Furthermore, EmbB has been shown to play a key role in forming the characteristic terminal hexarabinofuranosyl motif of AG, which is the template for mycolylation. Together with the other Emb proteins (EmbA and EmbC), EmbB belongs to the glycosyltransferase C (GT-C) superfamily, whose structures comprises an N-terminal transmembrane domain and a C-terminal soluble domain located on the periplasmic side of the membrane. EmbB is observed as a dimer along with an acyl-carrier-protein (AcpM) associated with each protomer, thus forming a heterotetrameric EmbB2-AcpM2 complex. The EmbB protomers in the two states share common structural features which include two periplasmic domains (PDs) and 15 transmembrane helices (TMH) arranged into an approximately crescent-shaped bundle.

In this study, we have determined the structures of a substrate unbound EmbB2-AcpM2 complex in a presumed resting state and a donor DPA-bound pre-catalytic conformation which we define as the “active” state. The EmbB2-AcpM2 complex is captured in two states, one with C2-symmetry and the other that is asymmetric. Given their differences in composition and conformation, the two states are referred to as the asymmetric “donor-bound” active state and the symmetric “resting” state. Another structural rearrangement upon DPA binding, by comparing the structures of the two states, involves α6 in PL5, a short α helix that interacts with DPA, whereas in the resting state, this region is disordered. Considering that the bound DPA is the major composition difference between the two states, it is reasonable to speculate that the dramatic structural rearrangement of the enzyme complex in the active state occurs upon DPA binding, and is mediated by the induced disorder-to-helix transition of α6 at the dimer interface. When superimposing the EmbB protomer from the EmbB2 in its resting state onto the EmbB subunit of ethambutol-bound EmbA-EmbB complex, residues including the catalytic site D285 on EmbB2 were obsereved in the similar position. Thus it is possible the ethambutol inhibition mode on EmbB2 similar to that on EmbA-EmbB complex by inhibiting substrate binding. Notable shifting (2.9~4.0 A°) were observed on E313 on PL2 and H580 on PL6, likely due to ethambutol binding.

>[2x]MSGNMDEAVSGNMDEAVSAGKDVRIARWVATIAGLLGFVLSVSIPLLPVTQTTATLNWPQQGRLDNVTAPLISQAPLELTATVPCSVVRDLPPEGGLVFGTAPAEGRDAALNAMLVNVTETRVDVIVRNVVVASVNRDRVAGPDCQRIEITSNLDGTYADFVGLTQISGEDAGKLQRTGYPDPNLRPAIVGVFTDLTGPAPQGLSVSAEIDTRFTTHPTALKLAAMLLAIVSTVIALLALWRLDRLDGRRMHRLIPTRWRTVTAVDGVVVGGMAIWYVIGANSSDDGYILQMARTAEHAGYMANYFRWFGSPEDPFGWYYNVLALMTKVSDASIWIRLPDLICALICWLLLSREVLPRLGPAVAGSRAAMWAAGLVLLGAWMPFNNGLRPEGQIATGALITYVLIERAVTSGRLTPAALAITTAAFTLGIQPTGLIAVAALLAGGRPILRIVMRRRRLVGTWPLIAPLLAAGTVILAVVFADQTIATVLEATRIRTAIGPSQEWWTENLRYYYLILPTTDGAISRRVAFVFTAMCLFPSLFMMLRRKHIAGVARGPAWRLMGIIFATMFFLMFTPTKWIHHFGLFAAVGGAMAALATVLVSPTVLRSARNRMAFLSLVLFVLAFCFASTNGWWYVSNFGAPFNNSVPKVGGVQISAIFFALSAIAALWAFWLHLTRRTESRVVDRLTAAPIPVAAGFMVVVMMASMAIGVVRQYPTYSNGWANIRAFAGGCGLADDVLVEPDSNAGFLTPLPGAYGPLGPLGGEDPQGFSPDGVPDRIIAEAIRLNNPQPGTDYDWNRPIKLDEPGINGSTVPLPYGLDPKRVPVAGTYSTEAQQESRLSSAWYELPARDETERAAHPLVVITAAGTITGESVANGLTTGQTVDLEYATRGPDGTLVPAGRVTPYDVGPTPSWRNLRYPRSEIPDDAVAVRVVAEDLSLSQGDWIAVTPPRVPELQSVQEYVGSDQPVLMDWAVGLAFPCQQPMLHANGVTEVPKFRISPDYYAKLQSTDTWQDGINGGLLGITDLLLRASVMSTYLSQDWGQDWGSLRKFDTVVEATPAELDFGSQTHSGLYSPGPLRIRP;>[2x]MAATQEEIIAGLAEIIEEVTGIEPSEVTPEKSFVDDLDIDSLSMVEIAVQTEDKYGVKIPDEDLAGLRTVGDVVAYIQKLEEENPEAAAALREKFAADQ>GEFMPQTFADAVAASLPHLRRYARALTGEQRTGDAIAARTLEGLIADPSVLERDLEPRLMLFRAFHRTWRREGAPVGEADSHLAQRAQSHLARLTPNTREALLLHAIEGFTAQEIGAVMEVPPETAADFIDTALREMAESVAGRVMIIEDEAIIAMDIAAIVREMGHRVTGIARTRFEAVRLAREERPDLILADIQLADNSSGIDAVNEILAEFADLPVIFITAFPERLLTGERPEP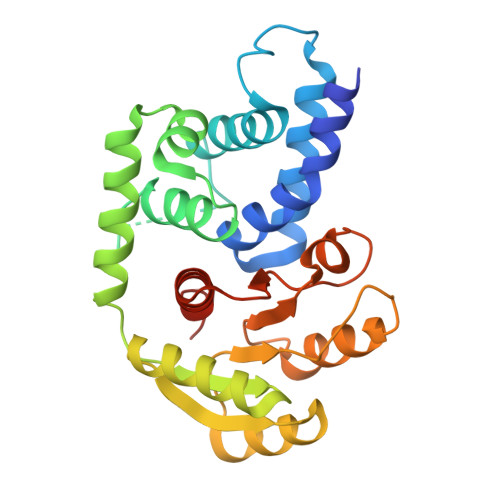AFLITKPYREEQVRSAVSQAMFFASTETLAA[4x]> QGRKIFKVFNQDFIVDERYTVTKELGQGAYGIVCAAVNNQTSEGVAIKKVTNVFSKKILAKRALREIKLLQHFRGHRNITCLYDMDIPRPDNFNETYLYEELMECDLAAIIRSGQPLTDAHFQSFIYQILCGLKYIHSANVLHRDLKPGNLLVNADCELKICDFGLARGFSVDPEENAGYMTEYVATRWYRAPEIMLSFQSYTKAIDVWSVGCIL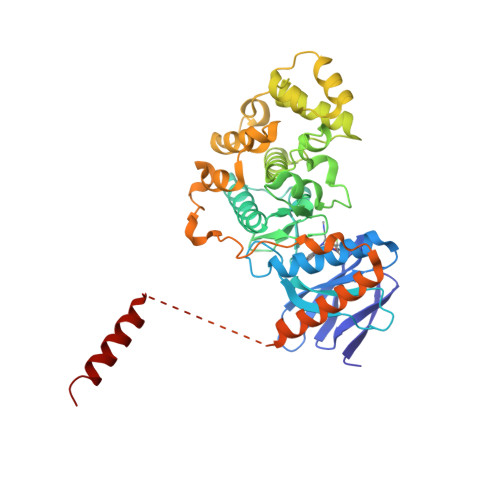AELLGGRPFFKGRDYVDQLNQILHILGTPNEETLSRIGSPRAQEYVRNLPFMAKKPFPTLFPNANPDALDLLDRMLAFDPSSRISVEQALEHPYLHIWHDASDEPDCPTTFNFDFEVVEDVGEMRKMILDEVYRFRQLVRTAPGAGGHGAPHAPQVPIPAGAGQGQWKAEDPRPQEYVGQMNDLEAELAGGLD>GHFVQQKVKVFRAADPLVGVFLWGVAHSINELSQVPPPVMLLPDDFKASSKIKVNNHLFHRENLPSHFKFKEYCPQVFRNLRDRFGIDDQDYLVSLTRNPPSESEGSDGRFLISYDRTLVIKEVSSEDIADMHSNLSNYHQYIVKCHGNTLLPQFLGMYRVSVDNEDSYMLVMRNMFSHRLPVHRKYDLKGSLVSREASDKEKVKELPTLKDMDFLNKNQKVYIGEEEKKIFLEKLKRDVEFLVQLKIMDYSLLLGIHDIIRGS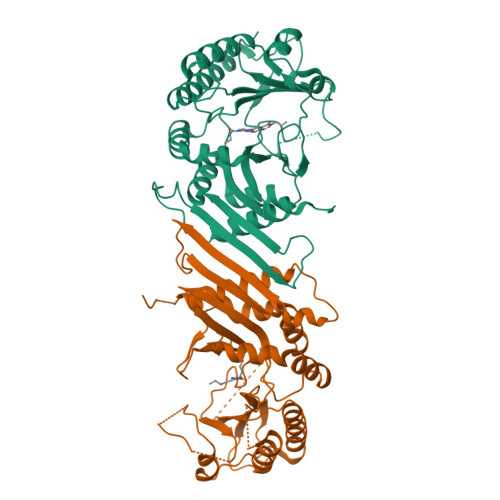EPEEELGPGEFESFIDVYAIRSAEGAPQKEVYFMGLIDILTQYDAKKKAAHAAKTVKHGAGAEISTVHPEQYAKRFLDFITNIFA[2x]> DADLATGAKVFSANCAACHAGGINLVNAEKTLKKEALEKFGMNSIVAITTVVTNGKAGMPAFKGRLTD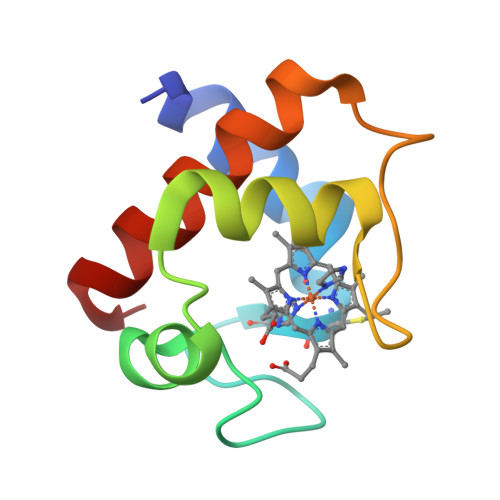DQIAAVAAYVLDQAEKGW> DGGYNAQLAKAKTELNEVSLAIKKSSMKMELLKKELLTIEPKLKEATKDNELNVKHVKQCQETCDKLRARLVEYGFDPSRIKDLKQREDKLKSHYYQTCKNSEYLKRRVTNLEFNYTKPYPNFEASFVHGVVGQLFQIDNDNIRYATALQTCAGGRLFNVVVQDSQTATQLLERGRLRKRVTIIPLDKIYTRPISSQVLDLAKKIAPGKVELAINLIRFDESITKAMEFIFGNSLICEDPETAKKITFHPKIRARSITLQGDVYDPEGTLSGGSRNTSESLLVDIQKYNQIQKQIETIQADLNHVTEELQTQYATSQKTKTIQSDLNLSLHKLDLAKRNLDANPSSQIIARNEEILRDIGECENEIKTKQMSLKKCQEEVSTIEKDMKEYDSDKGSK;> EKELEPWDLQLQEKESQIQLAESELSLLEETQAKLKKNVETLEEKILAKKTHKQELQDLILDLKKKLNSLKDERSQGEKNFTSAHLKLKEMQKVLNAHRQRAMEARSSLSKAQNKSKVLTALSRLQKSGRINGFHGRLGDLGVIDDSFDVAISTACPRLDDVVVDTVECAQHCIDYLRKNKLGYARFILLDRLRQFNLQPISTPENVPRLFDLVKPKNPKFSNAFYSVLRDTLVAQNLKQANNVAYGKKRFRVVTVDGKLIDISGTMSGGGNHVAKGLMKLGTNQSDKVDDYTPEEVDKIERELSERENNFRVASDTVHEMEEELKKLRD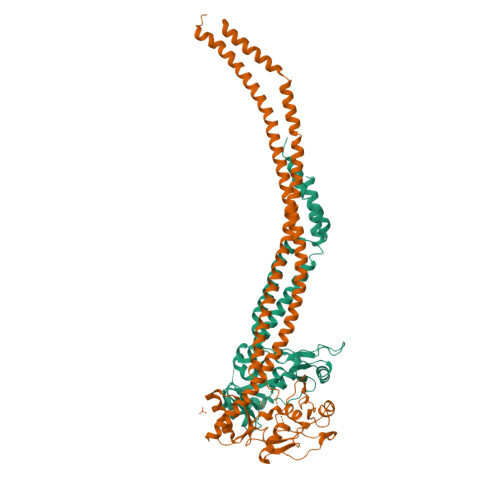HEPDLESQISKAEMEADSLASELTLAEQQVKEAEMAYVKAVSDKAQLNVVMKNLERLRGEYNDLQSE>QLPPSLPSDPRLWSREDVLVFLRFCVREFDLPKLDFDLFQMNGKRLCLLTRADFGHRCPGAGDVLHNVLQMLIIES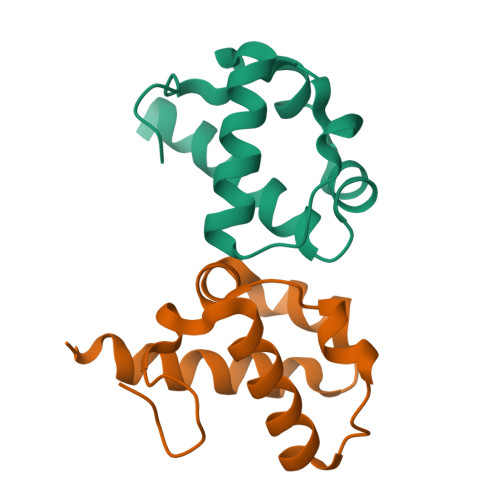HSRHHHHHH[2x];>PLGSDGLPLDPRDWTRADVWKWLINMAVSEGLEVTAELPQKFPMNGKALCLMSLDMYLCRVPVGGKMLYRDFRVRLARAMSR[2x]> M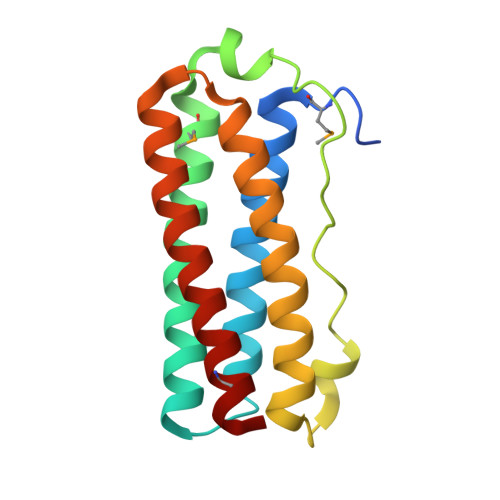GSDKIHHHHHHMKVSDILTVAIRLEEEGERFYRELSEHFNGEIKKTFLELADQERIHAEIFRKMSDQENWDEVDSYLAGYAFYEVFPDTSEILRRKDLTLKEVLDIAISVEKDSIILYYELKDGLVNSDAQKTVKKIIDQEKEHLRKLLEMKREST> MPLDPRIKKLLESGFVVPIGKASVDEVRKIFRQLASAAPKAEVRKVEDIKIPGSETSINARVYFPKAKGPYGVLVYLHGGGFVIGDVESYDPLCRAITNACNCVVVSVDYRLAPEYKFPSAVIDSFDATNWIYNNLDKFDGEMGIAIAGDSAGGNLAAV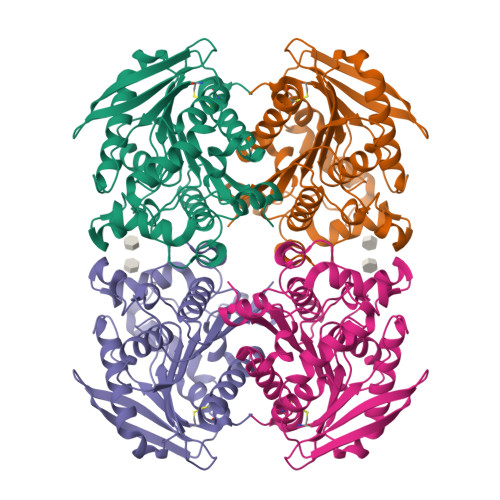VALLSKGKLDLKYQILIYPAVGFDSVSRSMIEYSDGFFLTREHIEWFGSQYLRSPADLLDFRFSPIIAQDLSGLPPALIITAEYDPLRDQGEAYANRLLQAGVPVTSVRFNNVIHGFLSFFPLIDQGKDAIGLIGSVLRRTFYDKS> MGSSHHHHHHSSGGDESQARVLHMVGDKPVFSFQPRGHLEIGEKLDIIRQKRLSHVSGHRSYYLRGAGALLQHGLVNFTFNKLLRRGFTPMTVPDLLRGAVFEGCGMTPNANPSQIYNIDPARFKDLNLAGTAEVGLAGYFMDH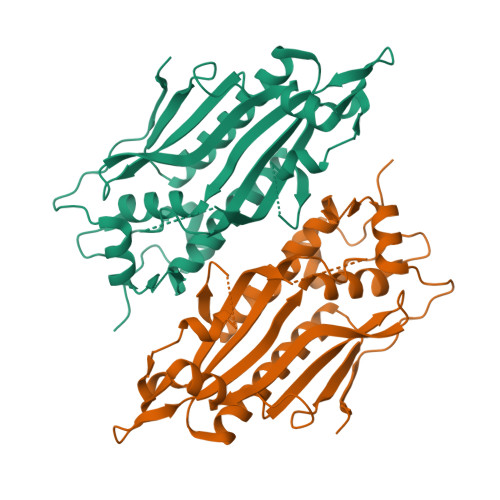TVAFRDLPVRMVCSSTCYRAETNTGQEPRGLYRVHHFTKVEMFGVTGPGLEQSSQLLEEFLSLQMEILTELGLHFRVLDMPTQELGLPAYRKFDIEAWMPGRGRFGEVTSASNCTDFQSRRLHIMFQTEAGELQFAHTVNATACAVPRLLIALLESNQQKDGSVLVPPALQSYLGTDRITAPTHVPLQYIGPNQPRKPGLPGQPAVS>[2x]MGSSHHHHH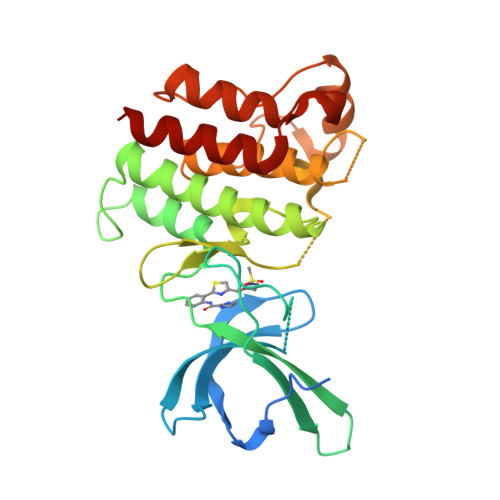HSSGLVPRGSSEELQNKLEDVVIDRNLLILGKILGEGEFGSVMEGNLKQEDGTSLKVAVKTMKLDNSSQREIEEFLSEAACMKDFSHPNVMRLLGVCIEMSSQGIPKPMVILPFMKYGDLHTYLLYSRLETGPKHIPLQTLLKFMVDIALGMEYLSNRNFLHRDLAARNCMLRDDMTVCVADFGLSKKIYSGDYYRQGRIAKMPVKWIAIESLADRVYTSKSDVWAFGVTMWEIATRGMTPYPGVQNHEMYDYLLHGHRLKQPEDCLDELYEIMYSCWRTDPLDRPTFSVLRLQLEKLLESLPDV>MGSSHHHHHHSQAPIEGRAQVINTFDGVADYLQTYHKLPDNYITKSEAQALGWVASKGNLCDVAPGKSIGGDIFSNREGKLPGKSGRTWREADINYTCGFRNSDRILYSSDWLIYKTTDHYQTFTKIR[3x];>MKKAVINGEQIRSISDLHQTLKKELALPEYYG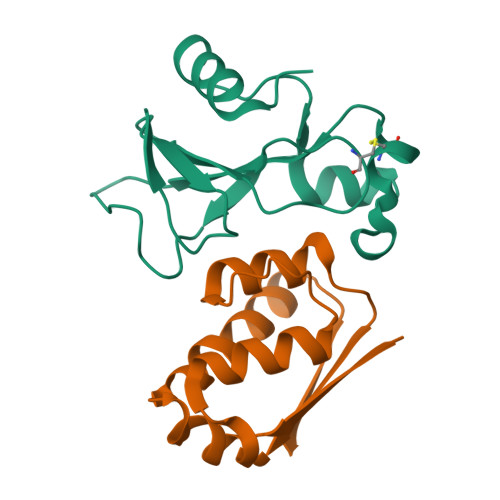ENLDALWDALTGWVEYPLVLEWRQFEQSKQLTENGAESVLQVFREAKAEGADITIILS[3x]>[5x]MRRAAMYEEGPPPSYESVVSAAPVAAALGSPFDAPLDPPFVPPRYLRPTGGRNSIRYSELAPLFDTTRVYLVDNKSTDVASLNYQNDHSNFLTTVIQNNDYSPGEASTQTINLDDRSHWGGDLKTILHTNMPNVNEFMFTNKFKARVMVSRLPTKDNQVELKYEWVEFTLPEGNYSETMTIDLMNNAIVEHYLKVGRQNGVLESDIGVKFDTRNFRLGFDPVTGLVMPGVYTNEAFHPDIILLPGCGVDFTHSRLSNLLGIRKRQPFQEGFRITYDDLEGGNIPALLDVDAYQASLKDDTEQGGGGAGGSNSSGSGAEENSNAAAAAMQPVEDMNDHAIRGDTFATRAEEKRAEAEAAAEAAAPAAQPEVEKPQKKPVIKPLTEDSKKRSYNLISNDSTFTQYRSWYLAYNYGDPQTGIRSWTLLCTPDVTCGSEQVYWSLPDMMQDPVTFRSTRQISNFPVVGAELLPVHSKSFYNDQAVYSQLIRQFTSLTHVFNRFPENQILARPPAPTITTVSENVPALTDHGTLPLRNSIGGVQRVTITDARRRTCPYVYKALGIVSPRVLSSRTF;>MKRARPSEDTFNPVYPYDTETGPPTVPFLTPPFVSPNGFQESPPGVLSLRLSEPLVTSNGMLALKMGNGLSLD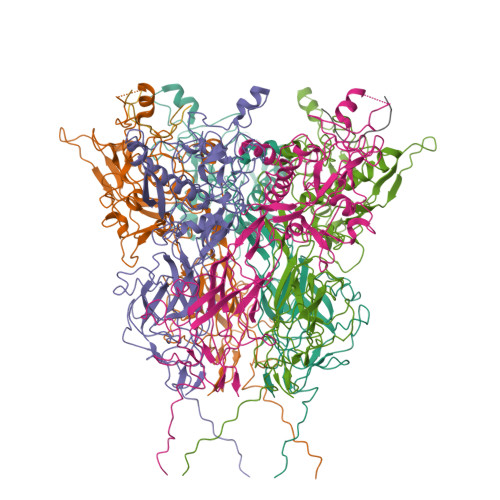EAGNLTSQNVTTVSPPLKKTKSNINLEISAPLTVTSEALTVAAAAPLMVAGNTLTMQSQAPLTVHDSKLSIATQGPLTVSEGKLALQTSGPLTTTDSSTLTITASPPLTTATGSLGIDLKEPIYTQNGKLGLKYGAPLHVTDDLNTLTVATGPGVTINNTSLQTKVTGALGFDSQGNMQLNVAGGLRIDSQNRRLILDVSYPFDAQNQLNLRLGQGPLFINSAHNLDINYNKGLYLFTASNNSKKLEVNLSTAKGLMFDATAIAINAGDGLEFGSLNAPNSNPLKTKIGHGLEFDSNKAMVPKLGTGLSFDSTGAITVGNKNNDKLTLWTTPAPSPNCRLNAEKDAKLTLVLTKCGSQILATVSVLAVKGSLAPISGTVQSAHLIIRFDENGVLLNNSFLDPEYWNFRNGDLTEGTAYTNAVGFMPNLSAYPKSHGKTAKSNIVSQVYLNGDKTKPVTLTITLNGTQETGDTTPSAYSMSFSWDWSGHNYINEIFATSSYTFSYIAQE[3x]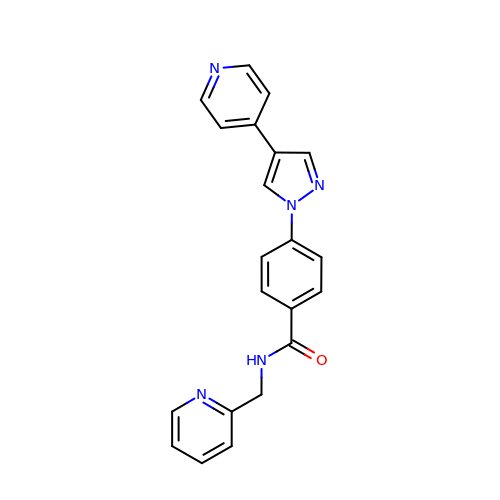N-[(pyridin-2-yl)methyl]-4-[4-(pyridin-4-yl)-1H-pyrazol-1-yl]benzamide | C21 H17 N5 O | UKGSBPKSNSXMDN-UHFFFAOYSA-N> DNPSYQQSPRHFVPTGMHSLALGTNLVEPLHALRLDAAGTTQHPVGCAPDEDMTVSSIASRYGLIRRVQWKKDHAKGSLLLQLDADPFVEQRIEGTNPISLYWFAPVGVVSSMFMQWRGSLEYRFDIIASQFHTGRLIVGYVPGLTASLQLQMDYMKLKSSSYVVF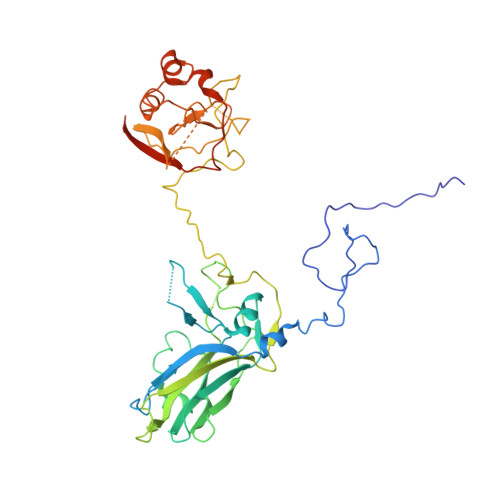DLQESNSFTFEVPYVSYRPWWVRKYGGNYLPSSTDAPSTLFMYVQVPLIPMEAVSDTIDINVYVRGGSSFEVCVPVQPSLGLNWNTDFILRNDEEYRAKTGYAPYYAGVWHSFNNSNSLVFRWGSASDQIAQWPTISVPRGELAFLRIKDGKQAAVGTQPWRTMVVWPSGHGYNIGIPTYNAERARQLAQHLYGGGSLTDEKAKQLFVPANQQGPGKVSNGNPVWEVMRAPLATQRAHIQDFEFIEAIPE>[2x]GVALGATRVIYPAGQKQEQLAVTNNDENSTYLIQSWVENADGVKDGRFIVTPPLFAMKGKKENTLRILDATNNQLPQDRESLFWMNVKAIPSMD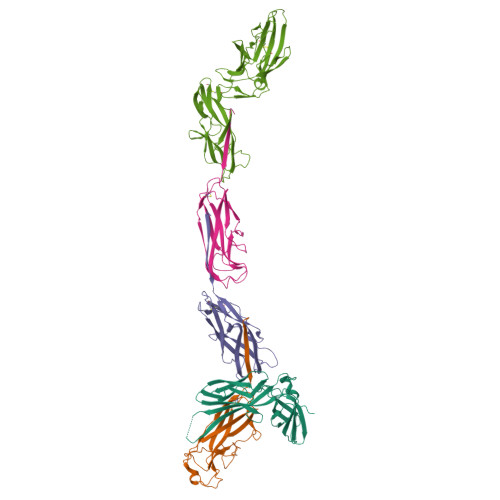KSKLTENTLQLAIISRIKLYYRPAKLALPPDQAAEKLRFRRSANSLTLINPTPYYLTVTELNAGTRVLENALVPPMGESTVKLPSDAGSNITYRTINDYGALTPKMTGVME;>ADSTITIRGYVRDNGCSVAAESTNFTVDLMENAAKQFNNIGATTPVVPFRILLSPCGNAVSAVKVGFTGVADSHNANLLALENTVSAAAGLGIQLLNEQQNQIPLNAPSSALSWTTLTPGKPNTLNFYARLMATQVPVTAGHINATATFTLEYQ[4x];>[2x]ADVTITVNGKVVAKPCTVSTTNATVDLGDLYSFSLMSAGAASAWHDVALELTNCPVGTSRVTASFSGAADSTGYYKNQGTAQNIQLELQDDSGNTLNTGATKTVQVDDSSQSAHFPLQVRALTVNGGATQGTIQAVISITYTYS;>[2x]FACKTANGTAIPIGGGSANVYVNLAPAVNVGQNLVVDLSTQIFCHNDYPETITDYVTLQRGSAYGGVLSSFSGTVKYNGSSYPFPTTSETPRVVYNSRTDKPWPVALYLTPVSSAGGVAIKAGSLIAVLILRQTNNYNSDDFQFVWNIYANNDVVVPTGGCDVSARDVTVTLPDYPGSVPIPLTVYCAKSQNLGYYLSGTTADAGNSIFTNTASFSPAQGVGVQLTRNGTIIPANNTVSLGAVGTSAVSLGLTANYARTGGQVTAGNVQSIIGVTFVYQ In low G + C Gram-positive bacteria, CodY is a global regulatory protein that controls the transcription of numerous genes. CodY from B. subtilis and most other low G + C Gram-positive bacteria is a DNA-binding protein that is activated by the branched-chain amino acids (BCAAs),2 leucine, isoleucine and valine, which may be viewed as signals of the metabolic status of the cell, and GTP, which may signal the energetic status of the cell. CodY from B. subtilis consists of 259 amino acid residues. The structures of full-length CodY from B. subtilis determined here reveal the effector binding domain and the DNA binding domain as discrete entities separated by a helical linker.

In addition, we have solved the structure of a leucine 3 to serine mutant, CodY(L3S), in complex with isoleucine at 3.0 Å resolution in a crystal form containing four molecules per asymmetric unit. Isoleucine was bound to the GAF domains of all four subunits in the CodY(L3S) tetramer. The ligand was almost completely enclosed in a pocket formed by the β2-β3 and β3-β4 segments of the polypeptide. This pocket is distal to the site of the leucine 3 to serine substitution that resides in helix α1 at the N terminus. The ligand carboxylate forms an ion pair with the side chain of Arg-61 and a further polar contact with the main chain amide of Val-100, whereas its amino group forms polar contacts to the main chain carbonyl groups of Thr-96 and Phe-98. The isobutyl side chain of the isoleucine ligand projects into the protein parallel to the β-sheet and is surrounded by the side chains of Met-62, Met-65, Phe-71, Pro-72, Tyr-75, and Pro-99. We conclude that ligand binding is essentially unchanged in CodY(L3S) and that the effects of the leucine 3 to serine mutation on the tertiary structure of the GAF domain are barely discernible. The domain topology of the isoleucine-bound CodY(L3S) tetramer is superficially similar to that of the unliganded wild-type form; however, the packing of the chains is significantly different. Following this superposition, it is apparent that isoleucine binding to CodY(L3S) is associated with displacements in the long α5 helix and a significant separation of the two wHTH domains in the dimer. For the Ile-bound CodY(L3S) structure, where splaying increases the translational and rotational separation of the recognition helices to 34 Å and 45°, a longer DNA recognition sequence of ∼30 bp would be needed.

>GSHMASLQKTRIINSMLQAAAGKPVNFKEMAETLRDVIDSNIFVVSRRGKLLGYSINQQIENDRMKKMLEDRQFPEEYTKNLFNVPETSSNLDINSEYTAFPVENRDLFQAGLTTIVPIIGGGERLGTLILSRLQDQFNDDDLILAEYGATVVGMEILREKAEEIEEEARSKAVVQMAISSLSYSELEAIEHIFEELDGNEGLLVASKIADRVGITRSVIVNALRKLESAGVIESRSLGMKGTYIKVLNNKFLIELENLKSH[4x]>TRPNHTIYINNLNEKIKKDELKKSLHAIFSRFGQILDILVSRSLKMRGQA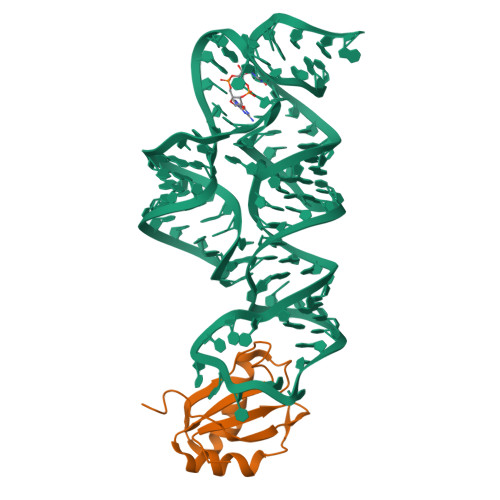FVIFKEVSSATNALRSMQGFPFYDKPMRIQYAKTDSDIIAK[2x]>[3x]MNPVTKQFQFGQSTVTLETGRIARQATGAVLVTMDDVSVLVTVVGAKSPAEGRDFFPLSVHYQEKTYAAGRIPGGFFKREGRPSEKETLTSRLIDRPIRPLFPEGFMNEVQVVCTVVSTNKKSDPDIAAMIGTSAALAISGIPFAGPIGAARVGFHPEIGYILNPTYEQLQSSSLDMVVAGTEDAVLMVESEADELTEDQMLGAVLFAHDEFQAVIRAVKELAAEAGKPAWDWKAPAENTVLVNAIKAELGEAISQAYTITIKQDRYNRLGELRDQAVALFAGEEEGKFPASEVKDVFGLLEYRTVRENIVNGKPRIDGRDTRTVRPLRIEVGVLGKTHGSALFTRGETQALVVATLGTARDAQLLDTLEGERKDAFMLHYNFPPFSVGECGRMGSPGRREIGHGRLARRGVAAMLPTQDEFPYTIRVVSEITESNGSSSMASVCGASLALMDAGVPVKAPVAGIAMGLVKEGEKFAVLTDILGDEDHLGDMDFKVAGTDKGVTALQMDIKINGITEEIMEIALGQALEARLNILGQMNQVIAKPRAELSENAP;> VPANATGRALNDPREKRRLQREAER

In Escherichia coli and numerous other bacteria, two of the principal enzymes mediating messenger RNA decay and RNA processing—RNase E, an endoribonuclease, and polynucleotide phosphorylase (PNPase), an exoribonuclease—assemble into a multi-enzyme complex known as the RNA degradosome. At the core of the assembly is the endoribonuclease RNase E, which initiates turnover of most messenger RNA (mRNA) transcripts and processes precursors of ribosomal RNAs, transfer RNAs, and small regulatory RNAs (sRNAs). Notwithstanding, PNPase predominantly acts as phosphorolytic 3′ → 5′ exoribonuclease that catalyses the processive degradation of single-stranded RNA, involved both in mRNA decay and sRNA-mediated gene regulation. Beyond the residues that form the catalytic core (1–529), each protomer of RNase E presents an intrinsically disordered C-terminal domain (CTD), extending from residues 530–1061, that serves as a scaffold for the RNA degradosome.

E. coli and P. aeruginosa are distant bacterial lineages, and their RNase E sequences differ significantly for the intrinsically disordered region and for the region corresponding to the identified binding sites for PNPase. To structurally investigate the interaction, the complex between the PNPase core and an MBP-tagged version of the C-terminal end of RNase E (883 – 1057) from P. aeruginosa was assembled and analysed by cryo-EM. The map reveals a new mode of interaction between the two ribonucleases, where a region of the intrinsically disordered part of RNase E from residues 948–964 interacts with the RNase PH domain of PNPase by the formation of an α-helix. The interaction is mediated by charged residues forming hydrogen bonds and salt bridges. Residues of the α-helix form several interactions with the backbone of the PNPase protomer, and one example is shown in the right panel of Fig. 4E. Moreover, two Arg residues form several salt bridges with negatively charged residues on the PNPase. Although the interacting area is smaller compared to what was found for E. coli and S. enterica, the number of interactions provides sufficient stability to be visualized by cryo-EM. Only a few residues forming the α-helix could be modelled due to poor resolution, suggesting high flexibility. We also structurally characterized the interaction between RNase E and PNPase in P. aeruginosa, revealing yet another mode of interaction involving the docking of the end of a long helix from RNase E to the surface of a PNPase protomer. The interaction between PNPase and RNase E in the pathogen P. aeruginosa has been reported to contribute to infective virulence and other complex phenotypes.> AAQTNAPWGLARISSTSPGTSTYYYDES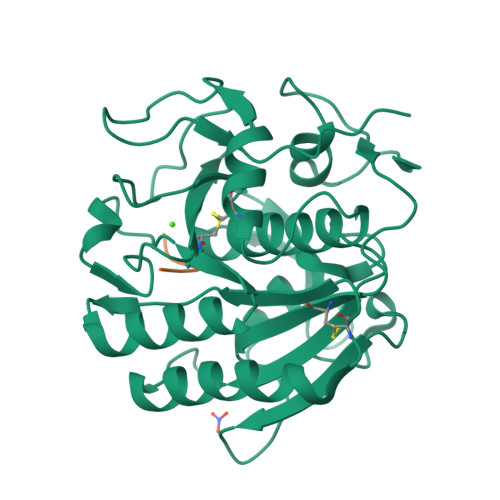AGQGSCVYVIDTGIEASHPEFEGRAQMVKTYYYSSRDGNGHGTHCAGTVGSRTYGVAKKTQLFGVKVLDDNGSGQYSTIIAGMDFVASDKNNRNCPKGVVASLSLGGGYSSSVNSAAARLQSSGVMVAVAAGNNNADARNYSPASEPSVCTVGASDRYDRRSSFSNYGSVLDIFGPGTDILSTWIGGSTRSISGTSMATPHVAGLAAYLMTLGKTTAASACRYIADTANKGDLSNIPFGTVNLLAYNNYQA;> LLFND>[4x]DPTMSVIKPDMKIKLRMEGAVNGHPFAIEGVGLGKPFEGKQSMDLKVKEGGPLPFAYDILTMAFCYGNRVFAKYPENIVDYFKQSFPEGYSWERSMIYEDGGICIATNDITLDGDCYIYEIRFDGVNFPANGPVMQKRTVKWEPSTEKLYVRDGVLKSDGNYALSLEGGGHYRCDSKTTYKAKKVVQLPDYHDVVHHIEIKSHDRDYSNVNLHEHAEAHSGLPRQAKX

Reversibly switchable fluorescent proteins (rsFPs) are essential tools in super-resolution imaging. The much smaller family of rsFPs exemplified by Padron are referred to as the positive switching rsFPs. Jakobs and co-workers demonstrated that only two mutations around the chromophore in Dronpa led to Padron, the prototype of a group of rsFPs in which the resting nonemissive off-state is the trans anionic form of the chromophore (trans−) which absorbs in the visible. In this work we apply ultrafast time resolved infrared (TRIR) along with TA and time resolved fluorescence (TRF) to characterise in detail the photodynamics in all three chromophore states (cis−, cisH, trans−) of the positive switching rsFP Kohinoor.

The structure of Kohinoor had not been reported. The chromophore structures are similar but not identical and there are also subtle differences in the wider structure. Comparing the two structures, the F176S mutation in Kohinoor reshapes the region around the chromophore. The loss of the bulky aromatic group apparently increases solvent accessibility and relaxes the steric bulk that contributes to the positioning of the neighboring Y162. The resulting shift in Y162 allows S145 to adopt a more favorable interaction with the chromophore, with a reduced hydrogen bond distance of 2.7 Å in Kohinoor, compared to 3.0 Å in Padron0.9, and a more favorable bond angle. The more open local environment also allows for additional conformational flexibility of the chromophore which can therefore adopt a slightly different conformation compared to Padron0.9 most notably in the methylene bridge region. Changes in that region are known to modify excited state dynamics in other FPs and in the bare chromophore. For example, the F176S mutation and the shifts in Y162 and S145 will change the protein environment around the phenolic OH, potentially suppressing ESPT in Kohinoor. Significantly, the cisH form of Kohinoor, which drives on- to off-state switching, was shown to behave very differently to the structurally and spectroscopically very similar Padron0.9, in that no ESPT reaction was observed in Kohinoor. This was assigned to small structural differences between Kohinoor and Padron which modify the environment of the phenolic group of the chromophore and to the different electrostatic environment and chromophore structure in the two proteins.> EPASTLEGPSRPVTVPLREDRGHAVDLPDTDPRVQRRVTGWAPEQIAVALSAAPTSAWVSWITGDFQMGGAVKPLDPGTVGSVVRYGLAADSLVREATGDALVYSQLYPFEGLQNYTSGIIHHVRLQGLEPGTKYYYQCGDPSIPGAMSAVHAFRTMPAVGPRSYPGRIAVVGDLGLTYNTTSTVEHMASNQPDLVLLLGDVSYANLYLTNGTGTDCYSCSFAKSTPIHETYQPRWDYWGRYMEPVTSSTPMMVVEGNHEIEQQIGNKTFAAYSARFAFPSMESESFSPFYYSFDAGGIHFIMLAAYADYSKSGEQYRWLEKDLAKVDRSVTPWLVAGWHAPWYSTYKAHYREAECMRVAMEELLYSYGLDIVFTGHVHAYERSNRVFNYTLDPCGAVHISVGDGGNREKMATTHADDPGRCPEPMSTPDAFMGGFCAFNFTSGPAAGSFCWDRQPDYSAYRESSFGHGILEVKNETHALWKWHRNQDLYQGAVGDEIYIVREPERCLLKHHHHHH

PAPs that can hydrolyze phytate are known as PAPhy (Dionisio et al., 2011). Here we show the X-ray crystal structure of the b2 isoform of wheat PAPhy induced during germination. In keeping with other HMW PAPs, TAPhy_b2 consists of a smaller fibronectin type III (FN3) non-catalytic N-terminal domain (residues Pro43–Thr156) together with a larger C-terminal MPE domain (residues Arg168–Glu497). The high-resolution crystal structures of the wheat purple acid phytase isoform b2 reported herein provide a straightforward explanation by highlighting the roles of two sequence inserts (PAPhy motifs) relative to a canonical MPE domain in forming phytate-specific substrate specificity pockets.

Crystals grown using glycoengineered recombinant protein diffracted only to low resolution, so the protein was enzymatically partially deglycosylated and repurified before crystallization. The resulting crystals grew in space group H3 and diffracted to 1.42 Å resolution. The refined crystal structure contains a monomer comprising residues Pro2-Leu508 of the 510-residue protein in the asymmetric unit. Four disulfide bonds and seven N-glycosylation sites are present, all according to previous predictions (Dionisio et al., 2011, 2012). A preference for Fe2+ in the MII site of the MPE domain has been described for TaPAPhy_b2 (Dionisio et al., 2011), a feature arising perhaps as a route to cellular redox regulation, and correspondingly two iron ions were modeled in the electron density present at the active site. Anomalous scattering peaks calculated using a dataset collected at the iron K-edge (Fe-SAD) supported this interpretation. X-ray fluorescence spectra combined with absorption edge scans confirmed the absence of manganese. The iron in the MI site is tetrahedrally coordinated by residues Asp174, Tyr204, His379, and Asp201, the latter of which bridges the two metal ions. The iron in the MII site is octahedrally coordinated by Asn258, His340, His377, and the bridging residue Asp201. A phosphate ion is bound to the two metal ions and the side chains of His259, His350, and Glu409.> MGSLGEEVQVIIVGLGIVGLAAAIECREKGHSVHAFEKSNILKSIGDCIGLQSNATRIIKRWGDGAVHEALRPWIVSSKEIRIHNSSGRLIIRQDLSEVCEQPNYLLPRSELIRVMYEHALKIGVEISLGVEVCEPSEDEEGASVVALTRDGERQIVRGDFIICSDGVHSKMRKAIMPQPVEPRPSGYAAFRALVDTETLKGDPEASWVFEGVEENDRFDVFFLSGAQIALQSCNKGKVFSWFCIHQDTRNLLDVWTSPADPNEMLDLIKVWPIGQRLWSVIRH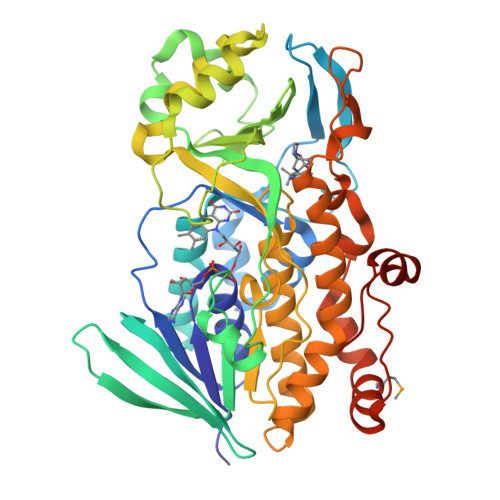TQPQKFINYPLLNHKPLDHWVSSHGRLILIGDAAHPLSPAAGQGASQGIEDANVLATSLSLAGRQRVSLALHVAERIRYARASAVQLISHRVNEGWRNQDWDAYEPNEQNIASLPLETWIYGHDSQAYTEQEFEMVVRAVQEGEEYHATNLPDKLRVQLGIRNVDVKEPLQNKSP Ena/VASP proteins form a family of cytoskeletal remodeling factors that are recruited to different regions of the cell by binding proline-rich SLiMs via their N-terminal EVH1 domains and promoting actin polymerization via their C-terminal EVH2 domains. The Ena/VASP EVH1 domain recognizes the SLiM [FWYL]PXΦP, where X is any amino acid and Φ is any hydrophobic residue. This motif, referred to in this paper as the FP4 motif, because FPPPP is a common example, adopts a polyproline type II (PPII) helix structure and binds weakly to the EVH1 domain. Focusing on the EVH1 domain of human ENAH, an actin regulator that is highly expressed in invasive cancers, we screened 36-residue proteome-derived peptides and discovered new interaction partners of ENAH and diverse mechanisms by which context influences binding.

A peptide from ENAH interactor ABI1 was among the highest affinity ligands that we validated by BLI, with KD = 2.6 μM. ABI1 contains an FP4 motif followed by four prolines. We solved a crystal structure of the ENAH EVH1-ABI1 peptide complex at 1.88 Å resolution. Only the FP8 region was fully resolved in the structure under the crystallization conditions, which included high salt and low pH. The peptide folds into a PPII helix with prolines 1, 4, and 7 (0FPPPPPPPP8) contacting the EVH1 surface. The FP4 portion of the peptide binds the canonical FP4 groove, as observed in other structures, whereas the 7th proline docks into a previously uncharacterized site on ENAH composed of Ala12, Gly92, Phe32, and the aliphatic part of the side chain of Asn90. We note that residue 12 has diverged in EVL and VASP EVH1 domains, which may contribute the weaker binding of ABI1 to those paralogs, although we have not isolated the affinity difference to this specific change. Notably, a similar binding site at the analogous location is used by the Homer EVH1 domain to bind the phenylalanine of PPXXF motifs. However, this site is relatively shallow in ENAH, and modeling large aromatic acids at this position on the ABI1 peptide using Pymol leads to severe steric clashes. Homer contains a smaller Gly89 at the site of Asn90 in ENAH and can accommodate the bulky Phe of the PPXXF motif.

> SNAMSEQSICQARAAVMVYDDANKKWVPAGGSTGFSRVHIYHHTGNNTFRVVGRKIQDHQVVINCAIPKGLKYNQATQTFHQWRDARQVYGLNFGSKEDANVFASAMMHALEVLGGSGSGFDDFPPPPPPPPVDYEDEEAAVVQYNDPYADGDPAW>[2x]GHHHHHHEFMHVFDNNGIELKAECSIGEEDGVYGLILESWGPGDRNKDYNIALDYIIERLVDSGVSQVVVYLASSSV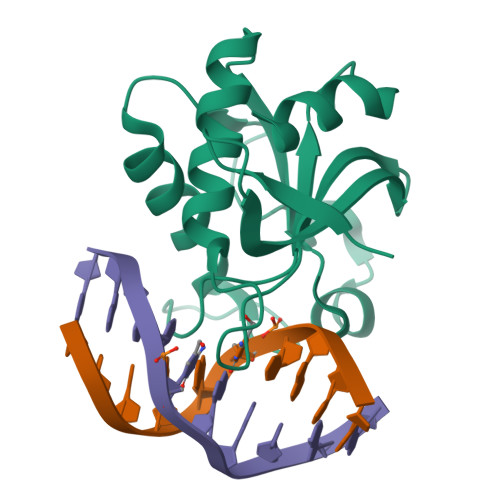RKHMHSLDERKIHPGEYFTLIGNSPRDIRLKMCGYQAYFSRTGRKEIPSGNRTKRILINVPGIYSDSFWASIIRG>MIISSLTNPNFKVGLPKVIAEVCDYLNTLDLNALENGRHDINDQIYMNVMEPETAEPSSKKAELHHEYLDVQVLIRGTENIEVGATYPNLSKYEDYNEADDYQLCADIDDKFTVTMKPKMFAVFYPYEPHKPCCVVNGKTEKIKKLVVKVPVKLI[4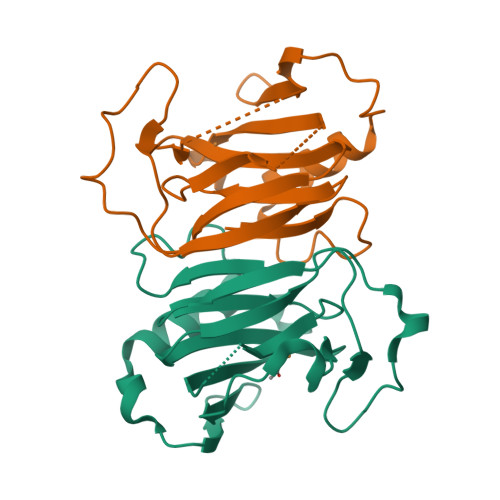x]> MHELTIYHFMSDKLNLYSDIGNIIALRQRAKKRNIKVNVV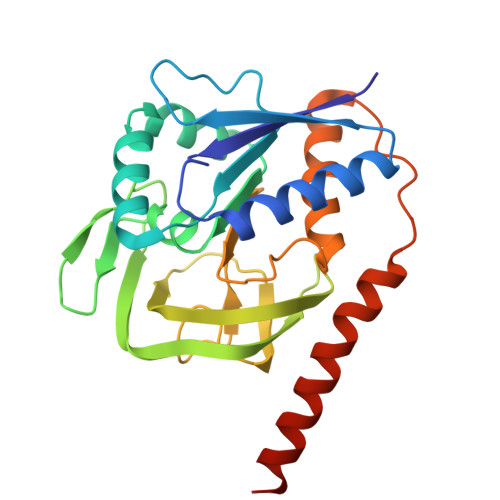EINETEGITFDECDIFFIGGGSDREQALATKELSKIKTPLKEAIEDGMPGLTICGGYQFLGKKYITPDGTELEGLGILDFYTESKTNRLTGDIVIESDTFGTIVGFENHGGRTYHDFGTLGHVTFGYGNNDEDKKEGIHYKNLLGTYLHGPILPKNYEITDYLLEKACERKGIPFEPKEIDNEAEIQAKQVLIDRANRQKKSRLEHHHHHH> HMSLSVANSTYETTALNSQKSSTDQPNSGSKSGQTLDLVNLGVAANFAILSKTGITDVYKSAITGDVGASPITGAAILLKCDEVTGTIFSVDAAGPACKITDASRLTTAVGDMQIAYDNAAGRLNPDFLNLGAGTIGGKTLTPGLYKWTSTLNIPTDITISGSSTDVWIFQVAGNLNMSSAVRITLAGGAQ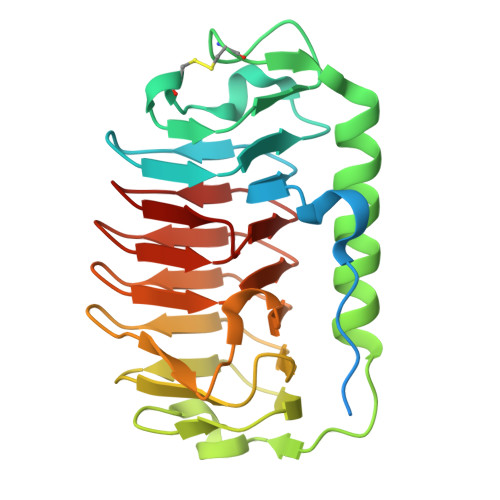AKNIFWQTAGAVTLGSTSHFEGNILSQTGINCKTAASINGRMMAQTAVTLQMCTVTIPQ> ADTIVAVELDSYPNTDIGDPSYPHIGIDIKSIRSKSTARWNMQTGKVGTAHISYNSVAKR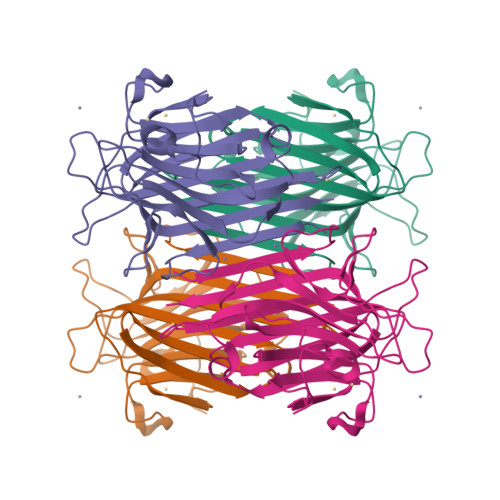LSAVVSYTGSSSTTVSYDVDLNNVLPEWVRVGLSATTGLYKETNTILSWSFTSKLKTNSIADANSLHFSFNQFSQNPKDLILQSDATTDSDGNLELTKVSSSGDPQGSSVGRALFYAPVHIWEKSAVVASFDATFTFLIKSPDRDPADGITFFIANTDTSIPSGSGGRLLGLFPDAN Segmented negative-strand RNA bunyaviruses encode a multi-functional polymerase that performs genome replication and transcription. Here, we establish conditions for in vitro activity of La Crosse virus polymerase and visualize its conformational dynamics by cryo-electron microscopy, unveiling the precise molecular mechanics underlying its essential activities. Replication initiation is performed de novo, in the absence of primer. Concerning transcription, LACV-L catalyses its initiation through a cap-snatching mechanism, whereby LACV-L steals cellular capped mRNA, binds them through its cap-binding domain (CBD), cleaves them 9 to 17 nucleotides downstream the cap with its endonuclease domain (ENDO), before using them as a primer for transcription initiation.

For the late-elongation state, a 5′-1-17BPm, 3′-vRNA-1-30 and four nucleotides were used. In this state, the 3′-vRNA is entirely replicated, a 10-base pair template-product duplex is visible in the active site and the 3′-vRNA end, following its exit from the active site as a single-stranded RNA, binds in the polymerase 3′-end secondary binding site. At late-elongation stage, the exit of the 3′ template from the template exit channel is coordinated with a repositioning of the vRBL and the clamp close to the core resulting in the formation of the 3′ secondary binding site as in pre-initiation. The replicated 3′-vRNA end exits as a single-stranded RNA from the active site cavity, binds to a positively charged groove, before reaching the 3′ secondary binding site, ready for the next replication cycle.

> MDYQEYQQFLARINTARDACVAKDIDVDLLMARKDYFGRELCKSLNIEYRNDVPFIDIILDIRPEVDPLTIDAPHITPDNYLYINNVLYIIDYKVSVSNESSVITYDKYYELTRDISDRLSIPIEIVIIRIDPVSRDLHINSDRFKELYPTIVVDINFNQFFDLKQLLYEKFGDDEEFLLKVAHGDFTLTAPWCKTGCPEFWKHPIYKEFKMSMPVPERRLFEESVKFNAYESERWNTNLVKIREYTKKDYSEHISKSAKNIFLASGFYKQPNKNEISEGWTLMVERVQDQREISKSLHDQKPSIHFIWGAHNPGNSNNATFKLILLSKSLQSIKGISTYTEAFKSLGKMMDIGDKAIEYEEFCMSLKSKARSSWKQIMNKKLEPKQINNALVLWEQQFMINNDLIDKSEKLKLFKNFCGIGKHKQFKNKMLEDLEVSKPKILDFDDANMYLASLTMMEQSKKILSKSNGLKPDNFILNEFGSRIKDANKETYDNMHKIFETGYWQCISDFSTLMKNILSVSQYNRHNTFRIAMCANNNVFAIVFPSADIKTKKATVVYSIIVLHKEEENIFNPGCLHGTFKCMNGYISISRAIRLDKERCQRIVSSPGLFLTTCLLFKHDNPTLVMSDIMNFSIYTSLSITKSVLSLTEPARYMIMNSLAISSNVKDYIAEKFSPYTKTLFSVYMTRLIKNACFDAYDQRQRVQLRDIYLSDYDITQKGIKDNRELTSIWFPGSVTLKEYLTQIYLPFYFNAKGLHEKHHVMVDLAKTILEIECEQRENIKEIWSTNCTKQTVNLKILIHSLCKNLLADTSRHNHLRNRIENRNNFRRSITTISTFTSSKSCLKIGDFRKEKELQSVKQKKILEVQSRKMRLANPMFVTDEQVCLEVGHCNYEMLRNAMPNYTDYISTKVFDRLYELLDKKVLTDKPVIEQIMDMMIDHKKFYFTFFNKGQKTSKDREIFVGEYEAKMCMYAVERIAKERCKLNPDEMISEPGDGKLKVLEQKSEQEIRFLVETTRQKNREIDEAIEALATEGSGWSHPQFEKGSGYESNLGKIEKLSLGKAKGLKMEINADMSKWSAQDVFYKYFWLIALDPILYPQEKERILYFMCNYMDKELILPDELLFNLLDQKVAYQNDIIATMTNQLNSNTVLIKRNWLQGNFNYTSSYVHSCAMSVYKEILKEAITLLDGSILVNSLVHSDDNQTSITIVQDKMENDKIIDFAMKEFERACLTFGCQANMKKTYVTNCIKEFVSLFNLYGEPFSIYGRFLLTSVGDCAYIGPYEDLASRISSAQTAIKHGCPPSLAWVSIAISHWMTSLTYNMLPGQSNDPIDYFPAENRKDIPIELNGVLDAPLSMISTVGLESGNLYFLIKLLSKYTPVMQKRESVVNQIAEVKNWKVEDLTDNEIFRLKILRYLVLDAEMDPSDIMGETSDMRGRSILTPRKFTTAGSLRKLYSFSKYQDRLSSPGGMVELFTYLLEKPELLVTKGEDMKDYMESVIFRYNSKRFKESLSIQNPAQLFIEQILFSHKPVIDFSGIRDKYINLHDSRALEKEPDILGKVTFTEAYRLLMRDLSSLELTNDDIQVIYSYIILNDPMMITIANTHILSIYGSPQRRMGMSCSTMPEFRNLKLIHHSPALVLRAYSKNNPDIQGADPTEMARDLVHLKEFVENTNLEEKMKVRIAMNEAEKGQRDIVFELKEMTRFYQVCYEYVKSTEHKIKVFILPAKSYTTTDFCSLMQGNLIKDKEWYTVHYLKQILSGGHKAIMQHNATSEQNIAFECFKLITHFADSFIDSLSRSAFLQLIIDEFSYKDVKVSKLYDIIKNGYNRTDFIPLLFRTGDLRQADLDKYDAMKSHERVTWNDWQTSRHLDMGSINLTITGYNRSITIIGEDNKLTYAELCLTRKTPENITISGRKLLGSRHGLKFENMSKIQTYPGNYYITYRKKDRHQFVYQIHSHESITRRNEEHMAIRTRIYNEITPVCVVNVAEVDGDQRILIRSLDYLNNDIFSLSRIKVGLDEFATIKKAHFSKMVSFEGPPIKTGLLDLTELMKSQDLLNLNYDNIRNSNLISFSKLICCEGSDNINDGLEFLSDDPMNFTEGEAIHSTPIFNIYYSKRGERHMTYRNAIKLLIERETKIFEEAFTFSENGFISPENLGCLEAVVSLIKLLKTNEWSTVIDKCIHICLIKNGMDHMYHSFDVPKCFMGNPITRDINWVMFREFINSLPGTDIPPWNVMTENFKKKCIALINSKFETQRDFSEFTKLMKKEGGRSNIEFD> EVPRKLLEEWLAMWSGHYQLKDKLRVQLRPQRAGSEVLELGIHGESDDKLANVIFQPIQDRRGRTILLVRDQNTFGAELRQKRLMTLIHLWLVHRFKAQAVHYVTPTDDNLYQTSKMKSHGIFTEVNQEVGEIIV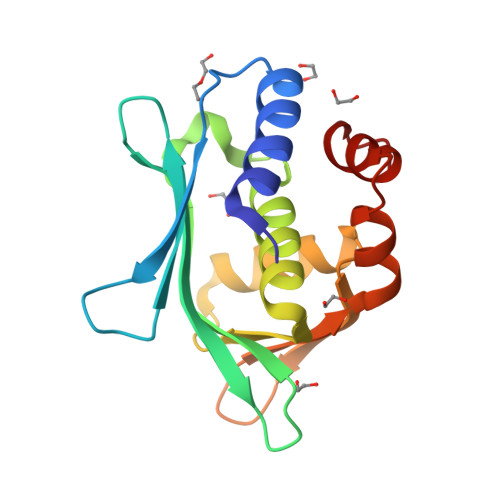AEVNHPRIAELLTPDRVALRKLITKEA> GAQVSSQKVGAHENSNRAYGGSTINYTTINYYKDSASNAASKQDY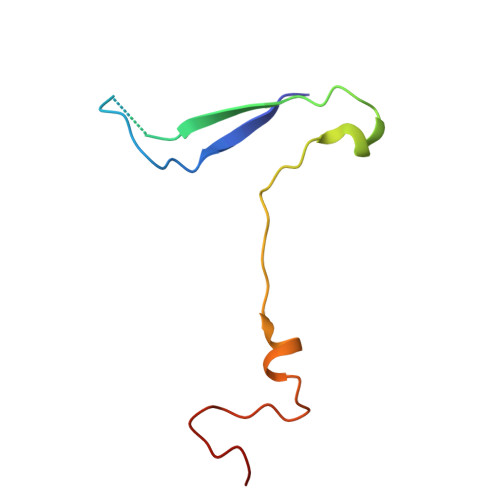SQDPSKFTEPLKDVLIKTAPALN> PGECSVNVIPKKNLDKAKFFSGTWYVTHYLDMDPQATEKFCFSFAPRESGGTVKEALYHFNVDSKVSFYNTG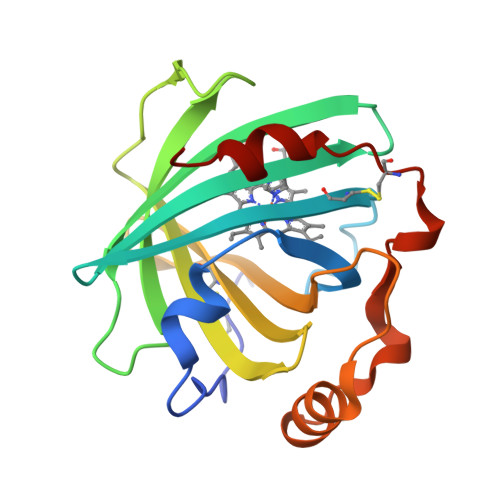TGPLESNGAKYTAKFNTVDKKGKEIKPADEKYSYTVTVIEAAKQSALIHICLQEDGKDIGDLYSVLNRNKNALPNKKIKKALNKVSLVLTKFVVTKDLDCKYDDKFLSSWQK> KETAAAKF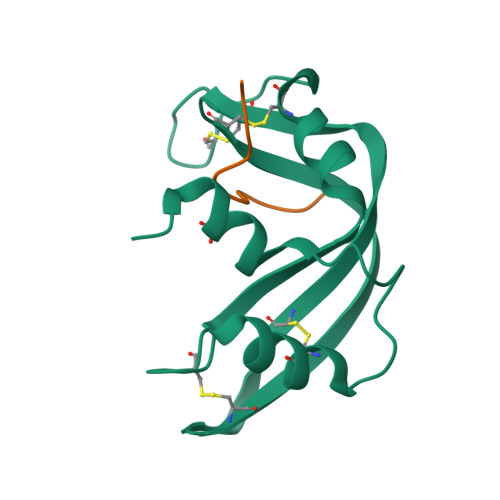ERQHMDSSTSAASSSNYCNQMMKSRNLTKDRCKPVNTFVHESLADVQAVCSQKNVACKNGQTNCYQSYSTMSITDCRETGSSKYPNCAYKTTQANKHIIVACEGNPYVPV;> EGSPYVPVHLDASV> GGSNSPDTANDGFVRLRGLPFGCSKEEIVQFFSGLEIVPNGMTLPVDFQGRSTGEAFVQFASQEIAEKA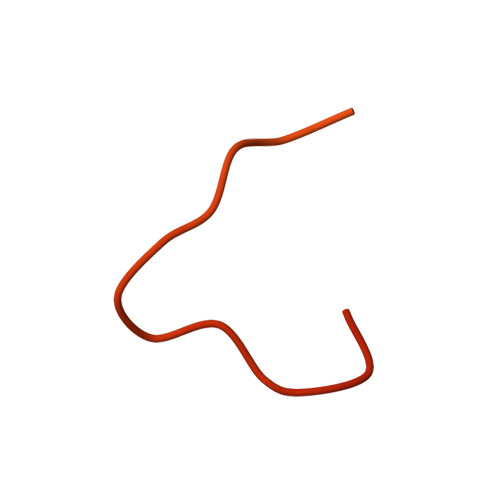LKKHKERIGHRYIEIFKSSRAEVRTHYDPPRKLMAMQRPGPYDRPGAGRGYNSIGRG> MALSTATKAATDALAANRAPTSVNAQEVHRWLQSFNWDFKNNRTKYATKYKMANETKEQFKLIAKEYARMEAVKDERQFGSLQDALTRLNAGVRVHPKWNETMK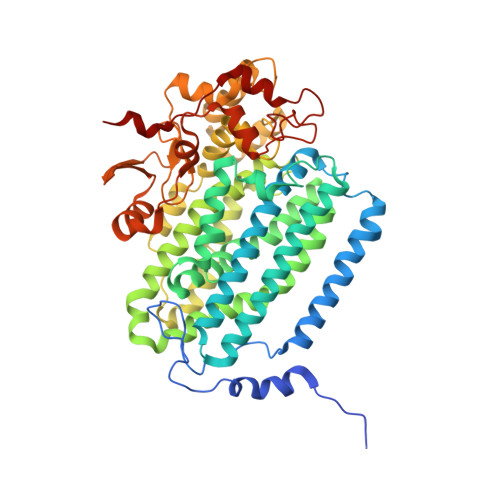VVSNFLEVGEYNAIAATGMLWDSAQAAEQKNGYLAQVLDEIRHTHQCAYVNYYFAKNGQDPAGHNDARRTRTIGPLWKGMKRVFSDGFISGDAVECSLNLQLVGEACFTNPLIVAVTEWAAANGDEITPTVFLSIETDELRHMANGYQTVVSIANDPASAKYLNTDLNNAFWTQQKYFTPVLGMLFEYGSKFKVEPWVKTWDRWVYEDWGGIWIGRLGKYGVESPRSLKDAKQDAYWAHHDLYLLAYALWPTGFFRLALPDQEEMEWFEANYPGWYDHYGKIYEEWRARGCEDPSSGFIPLMWFIENNHPIYIDRVSQVPFCPSLAKGASTLRVHEYNGEMHTFSDQWGERMWLAEPERYECQNIFEQYEGRELSEVIAELHGLRSDGKTLIAQPHVRGDKLWTLDDIKRLNCVFKNPVKAFN>[2x]NECISVKGRIYSILKQIGSGGSSKVFQVLNEKKQIYAIKYVNLEEADNQTLDSYRNEIAYLNKLQQHSDKIIRLYDYEITDQYIYMVMECGNIDLNSWLKKKKSIDPWERKSYWKNMLEAVHTIHQHGIVHSDLKPANFLIVDGMLKLIDFGIANQMQPDTTSVVKDSQVGTVNYMPPEAIKDMSSSRENGKSKSKISPKSDVW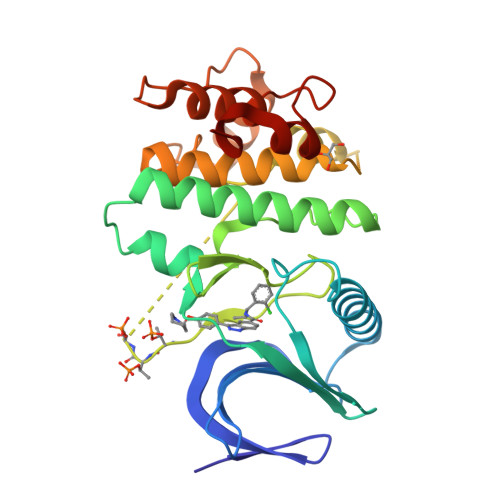SLGCILYYMTYGKTPFQQIINQISKLHAIIDPNHEIEFPDIPEKDLQDVLKCCLKRDPKQRISIPELLAHPYVQIQT> ANNLTFEAFEGIGQLNELNFYKYRLIGKGQIDNVHQAIWSVKYKLQANNFFKPVFVKGEILYSLDELKVIPEFENVEVILDGNIILSISENTDIYKDVIVFYINNALKNIKDITNYRKYITKNTDEIICKSILTTNLKYQYMKSEKGFKLQRKFKISPVVFRNGKVILYLNCSSDFSTDKSIYEMLNDGLGVVGLQVKNKWTNANGNIFIEKVLDNTISDPGTSGKLGQSLIDYYINGNQKYRVEKFTDEDKNAKVIQAKIKNKTYNYIPQALTPVITREYLSHTDKKFSKQIENVIKMDMNYRYQTLKSFVEDIGVIKELNNLHFKNQYYTNFDFMGFESGVLEEPVLMGANGKIKDKKQIFINGFFKNPKENVKFGVLYPEGCMENAQSIARSILDFATAGKYNKQENKYISKNLMNIGFKPSECIFESYKLGDITEYKATARKLKEHEKVGFVIAVIPDMNELEVENPYNPFKKVWAKLNIPSQMITLKTTEKFKNIVDKSGLYYLHNIALNILGKIGGIPWIIKDMPGNIDCFIGLAVGTREKGIHFPACSVLFDKYGKLINYYKPTIPQSGEKIAETILQEIFDNVLISYKEENGEYPKNIVIHRAGFSRENIDWYKEYFDKKGIKF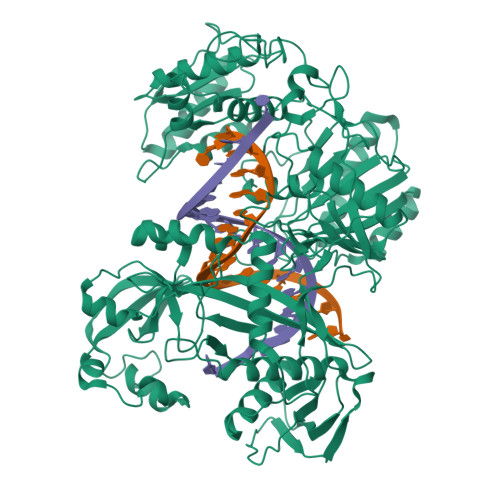NIIEVKKNIPVKIAKVVGSNICNPIKGSYVLKNDKAFIVTTDIKDGVASPNPLKIEKTYGDVEMKSILEQIYSLSQIHVGSTKSLRLPITTGYADKICKAIEYIPQGVVDNRLFFL Pyrazinamide (PZA), which is an analogue of nicotinamide, is an important first-line drug used in the short-course treatment of tuberculosis. PZA, which is a prodrug devoid of significant antibacterial activity, is metabolized into its active form, pyrazinoic acid (POA), by the amidase activity of the Mycobacterium tuberculosis nicotinamidase/pyrazinamidase (referred to as MtPncA), encoded by the pncA gene. The structure of PncA is made of a six-stranded parallel beta-sheet with helices packed on either side to form an α/β single domain. The substrate binding cavity in MtPncA is a small crevice of approximately 10 Å deep and 7 Å wide, which is delineated on one side by a catalytic triad made of residues Lys96 at the end of strand β3, Asp8 at the end of strand β1 and Cys138 at the N-ter extremity of helice α3.

The crystal structure of PncA was determined to 2.2 Å resolution by molecular replacement using PhPncA as search model. The asymmetric unit contained a single protein molecule. The metal ion present in PncA was finally identified by ICP-MS analysis, showing that MtPncA contained iron at a concentration of 180 µM for a total protein concentration of 260 µM in the assay. A final refinement considering Fe2+ as the ion present in PncA showed that the iron atom was coordinated in a distorted tetragonal bipyramidal arrangement by (i) the side chains of residues His51, His71 and two water molecules, HOH220 and 221 in equatorial position, and (ii) the side chains of Asp49 and His57 in axial position. Thus, our results are rather in agreement with the previous report of Zhang et al. who found that the M. tuberculosis pyrazinamidase contains iron and manganese with a molar ratio 1∶1, as opposed to what was speculated from the study of the pyrazinamidase of P. horikoshii which hypothesized that the metal ion present in PncA is a zinc playing a direct catalytic role by promoting a hydroxyl ion involved in hydrolysis of the drug. The latter assumption seems to be definitively ruled out considering the fact that the metal ion in MtPncA is located too far from the active site cysteine residue (Cys138) to be capable to contribute directly to PZA hydrolysis through the activation of a water molecule. Strikingly, and as opposed to previous observations made in PhPncA and AbPncA, the side chain of the key catalytic residue Cys138 in MtPncA was observed to be oriented not toward the centre of the binding cavity but, instead, toward the side chain of Lys96. The second striking structural feature observed in MtPncA corresponds to the very peculiar conformation of the 51–71 loop forming a protrusion that occludes the mouth of the binding cavity. Notably, His51 and His71 correspond to the hinge of the loop encompassing residues 52 to 70. This loop, which constitutes a flap closing the binding cavity, is locked by the third coordination bond established between His57 and Fe2+.

> MRALIIVDVQNDFCEGGSLAVTGGAALARAISDYLAEAADYHHVVATKDFHIDPGDHFSGTPDYSSSWPPHCVSGTPGADFHPSLDTSAIEAVFYKGAYTGAYSGFEGVDENGTPLLNWLRQRGVDEVDVVGIATDHCVRQTAEDAVRNGLATRVLVDLTAGVSADTTVAALEEMRTASVELVCSS PURINE 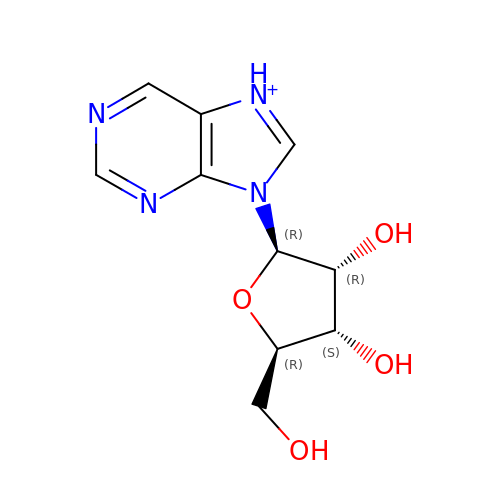RIBOSIDE | C10 H13 N4 O4 | MRWXACSTFXYYMV-FDDDBJFASA-O>PMTLGYWNIRGLAHSIRLLLEYTDSSYEEKKYTMGDAPDYDRSQWLNEKFKLGLDFPNLPYLIDGTHKITQSNAILRYIARKHNLCGESEKEQIREDILENQFMDSRMQLAKLCYDPDFEKLKPEYL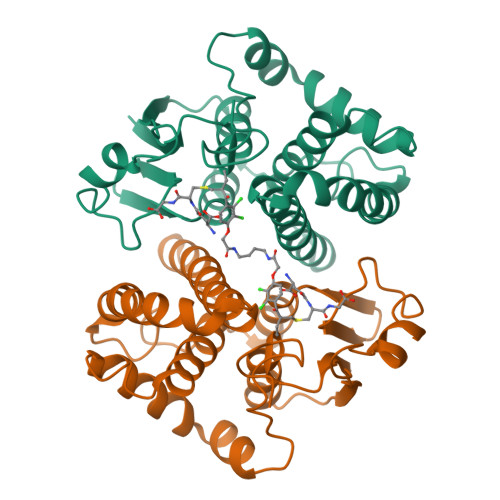QALPEMLKLYSQFLGKQPWFLGDKITFVDFIAYDVLERNQVFEPSCLDAFPNLKDFISRFEGLEKISAYMKSSRFLPRPVFTKMAVWGNK[2x]>[2x]GSSEHLKREHSLIKPYQGVGSSSMPLWDFQGSTILTSQYVRLTPDERSKEGSIWNHQPCFLKDWEMHVHFKVHGTGKKNLHGDGIALWYTRDRLVPGPVFGSKDNFHGLAIFLDTYPN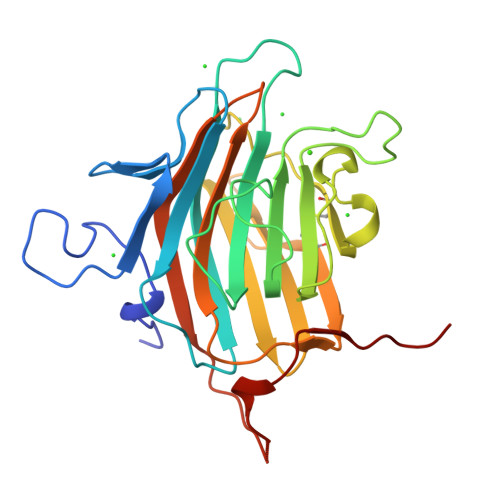DETTERVFPYISVMVNNGSLSYDHSKDGRWTELAGCTADFRNRDHDTFLAVRYSRGRLTVMTDLEDKNEWKNCIDITGVRLPTGYYFGASAGTGDLSDNHDIISMKLFQLMVEHTPDEENIDWTKIEPSVNFLKS> MGHHHHHHHHHHSSGHIDDDKHMVNVKKEFVDNMFSVKGKVALVTGATGALGCVLSKAYGYAGAKVFMTGRNEKKLQALEAEFKAEGIDCAYGVADPADEAQVDAMITACVAQYGEVNILAVTHGFNK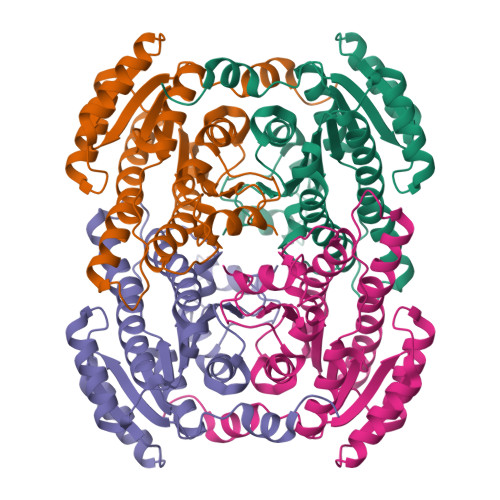PQNILEQSVADWQYIMDTDCKSVYVVCKYVAQQMVDQGKGGKIVVVTSQRSKRGMAGYTGYCTSKGGADLMVSSMACDLSAKYGINVNSICPTVFRSDLTEWMFDPESAVYQNFLKREPIGRLAEPEDFVGYALFLSSDASNYITGANCDCSGGYLTC;> MGHHHHHHHHHHSSGHIDDDKHMVNVKKEFVDNMFSVKGKVALVTGATGALGCVLSKAYGYAGAKVFMTGRNEKKLQALEAEFKAEGIDCAYGVADPADEAQVDAMITACVAQYGEVNILAVTHGFNKPQNILEQSVADWQYIMDADCKSVYVVCKYVAQQMVDQGKGGKIVVVTSQRSKRGMAGYTGYCTSKGGADLMVSSMACDLSAKYGINVNSICPTVFRSDLTEWMFDPESAVYQNFLKREPIGRLAEPEDFVGYALFLSSDASNYITGANCDCSGGYLTC>[2x]MANLHILSK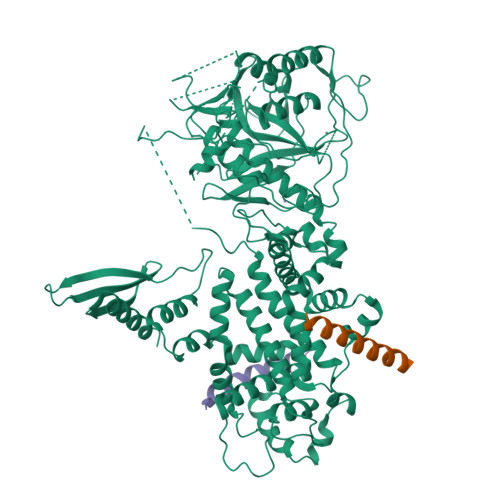LQEEMKRLAEEREETRHGGSRGDMLEVLFQ> GSMSKLIE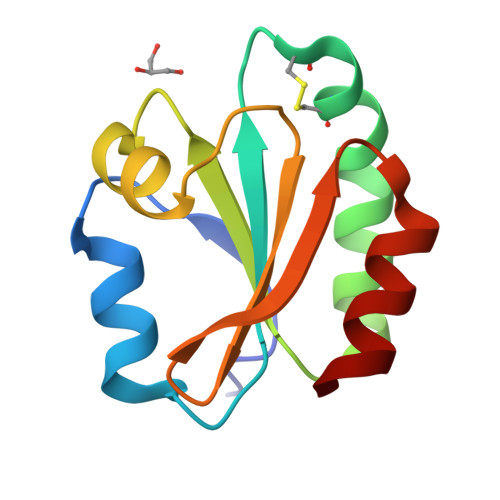LKQDGDLESLLEQHKNKLVVVDFFATWCGPCKTIAPLFKELSEKYDAIFVKVDVDKLEETARKYNISAMPTFIAIKNGEKVGDVVGASIAKVEDMIKKFI(3M)-3-(2-methyl-1H-imidazol-1-yl)pyridine | C9 H9 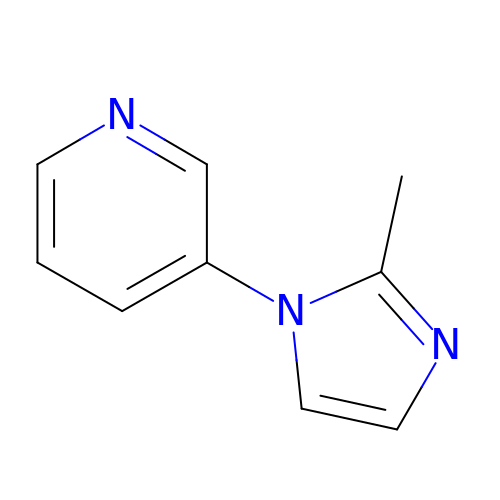N3 | MNHXJOCWNHZKLQ-UHFFFAOYSA-N> SFVDHPPDWLEEVGEGLREFLGLEAGPPKPKPNQQHQDQARGLVLPGYNYLGPGNGLDRGEPVNRADEVAREHDISYNEQLEAGDNPYLKYNHADAEFQEKLADDTSFGGNLGKAVFQAK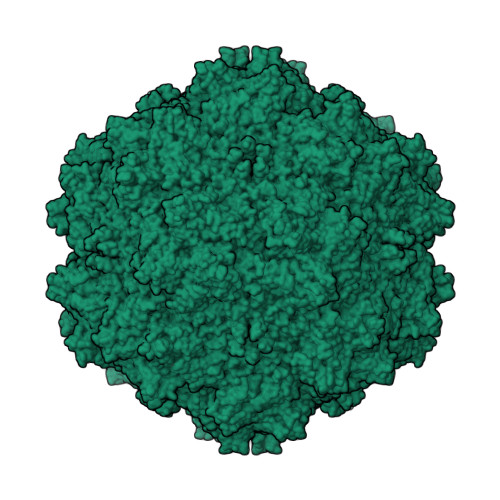KRVLEPFGLVEEGAKTAPTGKRIDDHFPKRKKARTEEDSKPSTSSDAEAGPSGSQQLQIPAQPASSLGADTMSAGGGGPLGDNNQGADGVGNASGDWHCDSTWMGDRVVTKSTRTWVLPSYNNHQYREIKSGSVDGSNANAYFGYSTPWGYFDFNRFHSHWSPRDWQRLINNYWGFRPRSLRVKIFNIQVKEVTVQDSTTTIANNLTSTVQVFTDDDYQLPYVVGNGTEGCLPAFPPQVFTLPQYGYATLNRDNTENPTERSSFFCLEYFPSKMLRTGNNFEFTYNFEEVPFHSSFAPSQNLFKLANPLVDQYLYRFVSTNNTGGVQFNKNLAGRYANTYKNWFPGPMGRTQGWNLGSGVNRASVSAFATTNRMELEGASYQVPPQPNGMTNNLQGSNTYALENTMIFNSQPANPGTTATYLEGNMLITSESETQPVNRVAYNVGGQMATNNQSSTTAPATGTYNLQEIVPGSVWMERDVYLQGPIWAKIPETGAHFHPSPAMGGFGLKHPPPMMLIKNTPVPGNITSFSDVPVSSFITQYSTGQVTVEMEWELKKENSKRWNPEIQYTNNYNDPQFVDFAPDSTGEYRTTRPIGTRYLTRPL3-[2-[2-[2-[2-[2-(2-azanylethoxy)ethoxy]ethoxy]ethoxy]ethoxy]ethoxy]propan-1-ol | C15 H33 N O7 | 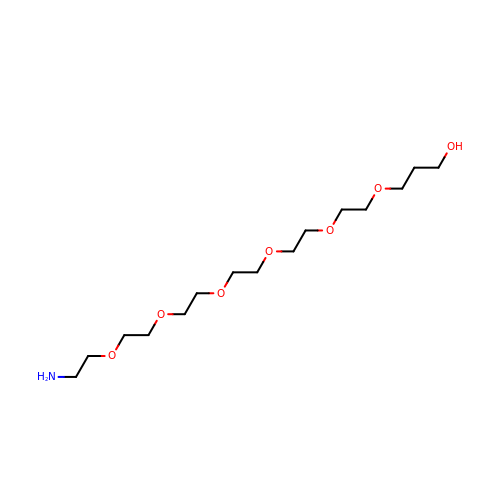ZSCFOXFWAAWAJH-UHFFFAOYSA-N>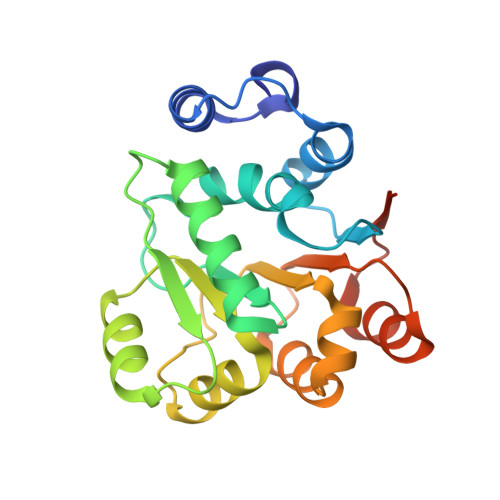 MQNFKELGISDNTVQSLESMGFKEPTPIQKDSIPYALQGIDILGQAQTGTGKTGAFGIPLIEKVVGKQGVQSLILAPTRELAMQVAEQLREFSRGQGVQVVTVFGGMPIERQIKALKKGPQIVVGTPGRVIDHLNRRTLKTDGIHTLILDEADEMMNMGFIDDMRFIMDKIPAVQRQTMLFSATMPKAIQALVQQFMKSPKIIKTMNNHHHHHH>MSRLDKSKVINSALELLNEVGIEGLTTRKLAQKLGVEQPTLYWHVKNKRALLDALAIEMLDRHHTHFSPLEGESWQDFLRNNAKSFRNALLSHRDGAKVHLGTRPTEKQYETLENQLAFLTQQGFSLENALYALSAVGHFTLGSVLEDQEHQVAKEERETPTTDSMPPLLRQAIELFDHQGAEPAFLHGLESLIRGFEVQLTALLQIV[2x]

Eponymous TetR is a homodimeric α-helical protein, and each monomer comprises 10 α-helices. The tertiary structure of TetR family members consists of two domains: an N-terminal nucleotide-binding domain (NBD) and a C-terminal effector-binding domain (EBD) that also contains the dimerization interface. In the absence of its natural ligand tc, TetR binds to the DNA tetO operator sequence and thereby represses downstream genes. Upon tc binding to the EBD, TetR undergoes an allosteric rearrangement that increases the separation of the NBDs, abolishes tetO operator binding and alleviates gene repression.

The apical GAAA tetraloop (nucleotides 22–25) could only be modelled in part. A crystal packing analysis suggested that no space is available for the placement of the central AA nucleotides. It is therefore possible that these nucleotides are absent in the crystal, most likely due to a random proteolytic degradation event. To further investigate this, a second TetR–aptamer complex was crystallized. The crystal structure of TetR in complex with a shortened 39-nucleotide-long TetR-binding RNA aptamer variant K2 was determined at 2.9 Å resolution. In this complex, nucleotides 2–37 could be modelled continuously, including the apical UUCG tetraloop of which the tip was missing in the previous structure. K2 shared 74% sequence identity with K1, and the overall fold of aptamer K2 was identical to that of aptamer K1. Apart from the fully formed apical tetraloop, the only two additional differences were a shortened 3 bp-long stem P1 and a likewise altered stem P2. Since all interactions between TetR and aptamer were identical in the K1 and K2 complexes and owing to the higher resolution of the TetR–RNA aptamer K1 complex, we limit ourselves to the description of the latter and refer to the K1 complex as the TetR–RNA aptamer complex from here on.>GSMGKDEALEKDLNDVSKEINLMLSTYAKLLSERAAVDASYIDEIDELFKEANAIENALIQKREELRQRF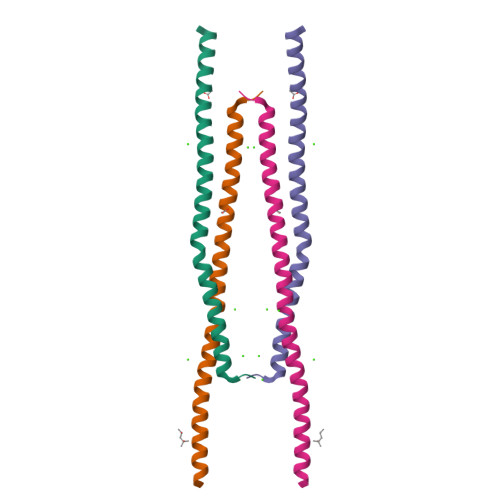TAIANTLHR[2x]2-[(3Z,6R)-6-[(2,6-dichlorophenyl)methyl]-3-(dimethylhydrazinylidene)-7-oxo-1,4-diazepan-1-yl]-N-[3-(1-methyl-1H-pyrazol-4-yl)phenyl]acetamide | C26 H29 Cl2 N7 O2 | 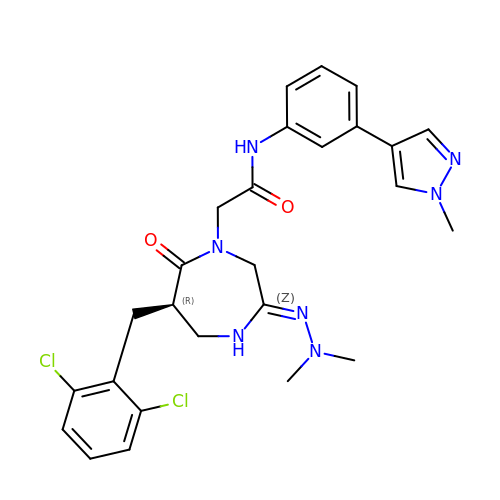GKZIYEBJQVXMQL-GOSISDBHSA-N>GAHMFKIPGFGKAAANHTPPDMTNMDTRTRHLKVSNCPNNSYALANVAAVSPNDFPNNIYIIIDNLFVFTTRHSNDIPPGTIGFNGNQRTWGGWSLNQDVQAKAFDLFKYSGKQSYLGSIDIDISFRARGKAVSTVFDQDELAKQFVRCYESQIFSPTQYLIMEFQGHFFDLKIRNVQAIDLGDIEPTSAVATGIETKGILTKQTQINFFKGRDGLVNLKSSNSLRPRSNAVIRPDFKFEDLGVGGLDKEFTKIFRRAFASRIFPPSVIEKLGISHVKGLLLYGPPGTGKTLIARKIGTMLNAKEPKIVNGPEILSKYVGSSEENIRNLFKDAEAEYRAKGEESSLHIIIFDELDSVFKQRGSRGDGTGVGDNVVNQLLAKMDGVDQLNNILVIGMTNRKDLIDSALLRPGRFEVQVEIHLPDEKGRLQIFDIQTKKMRENNMMSDDVNLAELAALTKNFSGAEIEGLVKSASSFAINKTVNIGKGATKLNTKDIAKLKVTREDFLNALNDVTPAFGISEEDLKTCVEGGMMLYSERVNSILKNGARYVRQVRESDKSRLVSLLIHGPAGSGKTALAAEIALKSGFPFIRLISPNELSGMSESAKIAYIDNTFRDAYKSPLNILVIDSLETLVDWVPIGPRFSNNILQMLKVALKRKPPQDRRLLIMTTTSAYSVLQQMDILSCFDNEIAVPNMTNLDELNNVMIESNFLDDAGRVKVINELSRSCPNFNVGIKKTLTNIETARHDEDPVNELVELMTQSA[6x];>[2x]GMSDPVELLKRAEKKGVPSSGFMKLFSGSDSYKFEEAADLCVQAATIYRLRKELNLAGDSFLKAADYQKKAGNEDEAGNTYVEAYKCFKSGGNSVNAVDSLENAIQIFTHRGQFRRGANFKFELGEILENDLHDYAKAIDCYELAGEWYAQDQSVALSNKCFIKCADLKALDGQYIEASDIYSKLIKSSMGNRLSQWSLKDYFLKKGLCQLAATDAVAAARTLQEGQSEDPNFADSRESNFLKSLIDAVNEGDSEQLSEHCKEFDNFMRLDKWKITILNKIKESIQQQEDDLL;> GASHMSSSTPFDPYALSEHDEERPQNVQSKSRTAELQAEIDDTVGIMRDNINKVAERGERLTSIEDKADNLAVSAQGFKRGANRVRKAMWYKDLKMK;> GASHMSYNNPYQLETPFEESYELDEGSSAIGAEGHDFVGFMNKISQINRDLDKYDHTINQVDSLHKRLLTEVNEEQASHLRHSLDNFVAQATDLQFKLKNEIKSAQRDGIHDTNKQAQAENSRQRFLKLIQDYRIVDSNYKEENKEQAKRQYMIIQPEATEDEVEAAISDVGGQQIFSQALLNANRRGEAKTALAEVQARHQELLKLEKSMAELTQLFNDMEELVIEQQENVDVIDKNVEDAQLDVEQGVGHTDKAVKSARKARKNKIR;> GASHIKFTKQSSVASTRNTLKMAQDAERAGMNTLGMLGHQSEQLNNVEGNLDLMKVQNKVADEKVAELKKLNRSILAVHVSNPFNSKRRRREREEQLKNRKIEEKLMREQTSQQLSQSTQRIEGAMNANNNISEVRERYQRKNVLEKAKRYQFENDEEDDEMELEIDRNLDQIQQVSNRLKKMALTTGKELDSQQKRLNNIEESTDDLDINLHMNTNRLAGI

SNARE (soluble N-ethylmaleimide-sensitive factor (NSF) attachment protein receptor) proteins drive membrane fusion at different cell compartments as their core domains zipper into a parallel four-helix bundle. After fusion, these bundles are disassembled by the AAA+ (ATPase associated with diverse cellular activities) protein Sec18/NSF and its adaptor Sec17/α-SNAP to make them available for subsequent rounds of membrane fusion. The disassembly requires multiple ATP hydrolysis events in the presence of Mg2+; as few as six ATP hydrolysis events are sufficient. The side-loading and side-release mechanism explains how Sec18/NSF can disassemble SNAREs with constrained topologies.

We present cryo-electron microscopy (cryo-EM) structures of a yeast SNARE complex, Sec18 and Sec17 in a nonhydrolyzing condition, which show SNARE Sso1 threaded through the D1 and D2 ATPase rings of Sec18, with its folded, N-terminal Habc domain interacting with the D2 ring. We chose the Sso1–Sec9–Snc1/Snc2 complex (referred to as the ySNARE complex) because each component of this complex crosslinked with high confidence to the D2 domain of Sec18 (Snc1 is highly homologous to Snc2). We prepared the y20S complex in a nonhydrolyzing condition and, after single-particle cryo-EM data collection and processing, we obtained 381,591 high-quality particles that yielded eight three-dimensional (3D) classes into which models were built. In the structures of all eight classes, Sso1 is threaded through the D1 pore of Sec18. Remarkably, our cryo-EM structures revealed that Sso1 is loaded into both the D1 and the D2 pores because the Habc domain of Sso1 interacts with the outside of the D2 ring, with class 1 having the most well-defined, discrete density. In class 1, the density for Sso1 within Sec18 is continuous from the D1 pore entrance to the D2 pore exit, where the Habc domain begins. The three-helix bundle of the Habc domain is then positioned outside the D2 pore, where it packs between two small D2 subdomains (protomers A and B) in an interaction driven by charge complementarity. Indeed, the electrostatic potential surface of the Habc domain forms a roughly opposite that of the bottom of the D2 surface against which it packs. Given that this charge distribution is replicated between each pair of D2 subdomains around the D2 surface, it is unsurprising that the Habc domain adopts multiple corresponding rotational states over the eight classes, presumably because of the flexible linker that follows it. This structural observation is consistent with XL-MS data showing a crosslink between the Habc and the D2 domain of Sec18. The nucleotide states and the arrangements of D1 around the substrate were also the same among all eight classes, with the ADP-engaged E protomer forming the top of a spiral staircase of tyrosine residues.>MPASQDKLDVPPGPYHFSEQVGHLLRRAYQRHVAIFQQTIPDSKLTAAQFVVLCALRDQGACSLVDVVKATAIDQATVRGVIERLKARKLLAVSHDPADRRKVLVTLTPDGRALVEEMVPFAEQITQSTFGGLNPAERVAIVYLLRKMSDADDLVG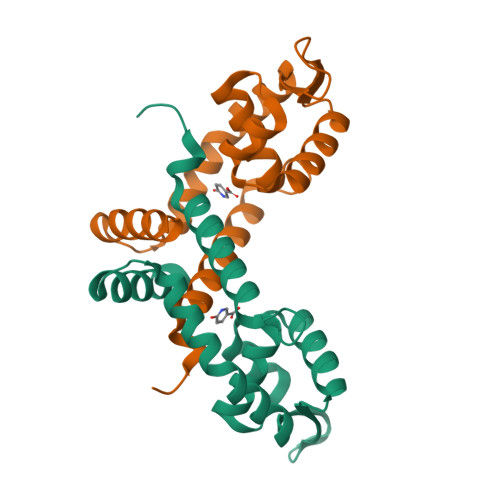RQSDS[6x]> MAELRVLVAVKRVIDYAVKIRVKPDRTGVVTDGVKHSMNPFCEIAVEEAVRLKEKKLVKEVIAVSCGPAQCQETIRTALAMGADRGIHVEVPPAEAERLGPLQVARVLAKLAEKEKVDLVLLGKQAIDDDCNQTGQMTAGFLDWPQGTFASQVTLEGDKLKVEREIDGGLETLRLKLPAVVTADLRLNEPRYATLPNIMKAKKKKIEVIK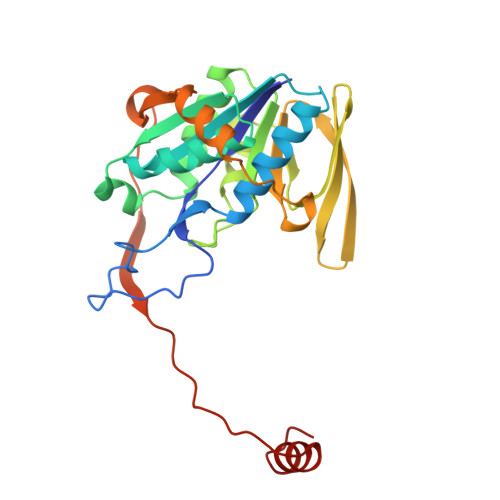PGDLGVDLTSKLSVISVEDPPQRTAGVKVETTEDLVAKLKEIGRI> METKYELNNTKKVANAFGLNEEDTNLLINAVDLDIKNNMQEISSELQQSEQSKQKQYGTTLQNLAKQNRII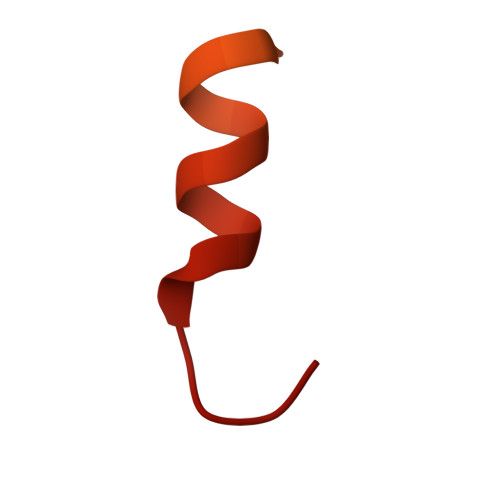K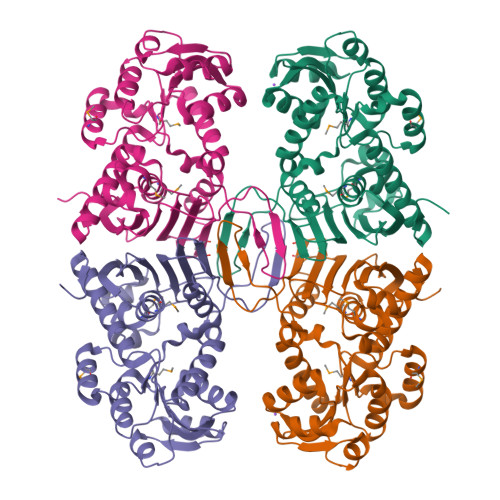>MSLTLRIALFGAGRIGHVHAANIAANPDLELVVIADPFIEGAQRLAEANGAEAVASPDEVFARDDIDGIVIGSPTSTHVDLITRAVERGIPALCEKPIDLDIEMVRACKEKIGDGASKVMLGFNRRFDPSFAAINARVANQEIGNLEQLVIISRDPAPAPKDYIAGSGGIFRDMTIHDLDMARFFVPNIVEVTATGANVFSQEIAEFNDYDQVIVTLRGSKGELINIVNSRHCSYGYDQRLEAFGSKGMLAADNIRPTTVRKHNAESTEQADPIFNFFLERYDAAYKAELATFAQGIRDGQGFSPNFEDGVIALELANACLESAQTGRTVTLNPANEGHHHHHH[4x]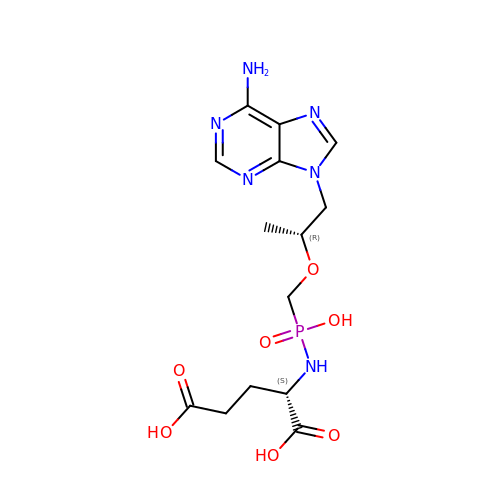L-Glutamate Tenofovir | C14 H21 N6 O7 P | CIXAAKVRZFPIJB-BDAKNGLRSA-N2-(3-phenoxyphenyl)-N-[5-[[(3R)-1-pyridazin-3-ylpyrrolidin-3-yl]amino]-1,3,4-thiadiazol-2-yl]ethanamide | C24 H23 N7 O2 S 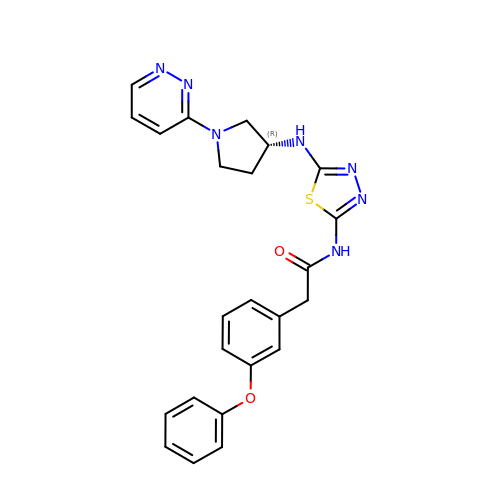| JOKJBMFEUFULOX-GOSISDBHSA-N>[3x]MGSDK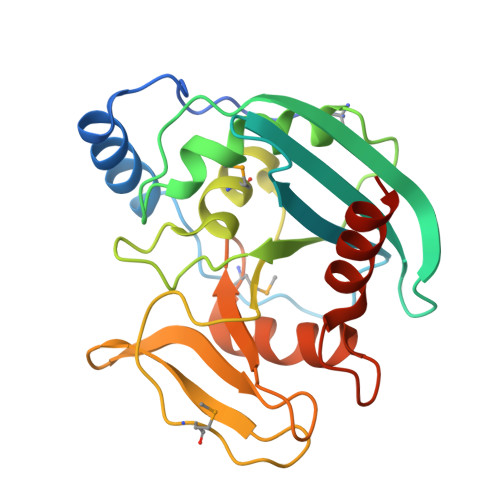IHHHHHHMDYRQLHRWDLPPEEAIKVQNELRKKIKLTPYEGEPEYVAGVDLSFPGKEEGLAVIVVLEYPSFKILEVVSERGEITFPYIPGLLAFREGPLFLKAWEKLRTKPDVVVFDGQGLAHPRKLGIASHMGLFIEIPTIGVAKSRLYGTFKMPEDKRCSWSYLYDGEEIIGCVIRTKEGSAPIFVSPGHLMDVESSKRLIKAFTLPGRRIPEPTRLAHIYTQRLKKGLF> XSEAAAS;> MLF;>[2x]HGSPVDICTAKPRDIPMNPMCIYRSPEKKATEDEGSEQKIPEATNRRVWELSKANSRFATTFYQHLADSKNDNDNIFLSPLSISTAFAMTKLGACNDTLQQLMEVFKFDTISEKTSDQIHFFFAKLNCRLYRKANKSSKLVSANRLFGDKSLTFNETYQDISELVYGAKLQPLDFKENAEQSRAAINKWVSNKTEGRITDVIPSEAINELTV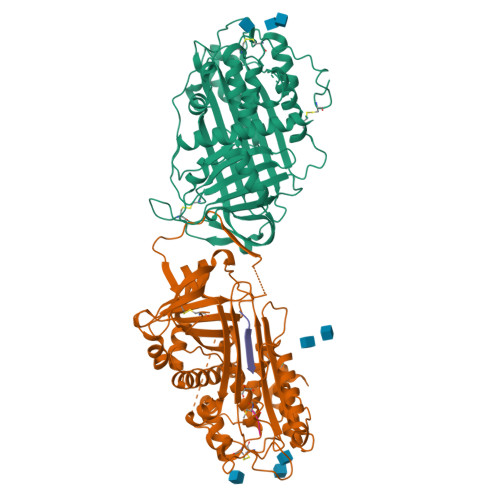LVLVNTIYFKGLWKSKFSPENTRKELFYKADGESCSASMMYQEGKFRYRRVAEGTQVLELPFKGDDITMVLILPKPEKSLAKVEKELTPEVLQEWLDELEEMMLVVHMPRFRIEDGFSLKEQLQDMGLVDLFSPEKSKLPGIVAEGRDDLYVSDAFHKAFLEVNEEGSEAAASTAVVIAGRSLNPNRVTFKANRPFLVFIREVPLNTIIFMGRVANPCVK The replication of positive-strand RNA viruses relies on virally encoded RNA-dependent RNA polymerases (RdRPs) that are capable of rapid and processive synthesis of the 7–14 kilobase viral genomes. To examine this in further detail and to validate the polymerase–RNA interactions seen in the initial poliovirus EC structures, we here present nine new coxsackievirus, rhinovirus, and poliovirus elongation complex structures at resolutions ranging from 2.1 to 2.9 Å. All the complexes feature an upstream RNA duplex that is pinched between the pinky finger and thumb domains such that the RNA exit channel is opened by ≈4 Å as compared to the polymerase alone structures. All of the complexes show the open conformation for the active site wherein the β-strands of motifs A and C are not hydrogen bonded together to fully form the RMM-fold that is commonly utilized by polymerase active sites.

Using this r2 RNA, we were able to obtain crystals of the CV polymerase EC under two conditions but in the same crystal form, resulting in a 2.4 Å resolution structure (CV_r2) and a 2.2 Å resolution structure (CV_r2_Mg) that clearly showed a Mg2+ ion pre-bound to the coxsackievirus polymerase EC in the absence of an added NTP. In the CV_r2_Mg structure we observe clear density for a six-fold coordinated magnesium ion bound to the polymerase at a site about 5 Å away from the active site itself. This is at a site that is commonly occupied by divalent metals in a number of other structures of the polymerase alone, and in several of the EC structures presented here the site is occupied by what is either a magnesium ion or a water molecule. In the CV_r2_Mg structure we see clear density for a bound magnesium ion that is coordinated by Asp330 in motif C and five water molecules in a six-fold coordination geometry, with Asp233 from motif A being involved in the network. This magnesium ion likely represents the polymerase bound Metal A ion that is moved into the active site to facilitate catalysis in conjunction with the Metal B magnesium that is brought in with the NTP, and it is bound in site where metals have been observed in several other viral polymerase structures even in the absence of RNA and NTPs.

>[4x]GEIEFIESSKDAGFPVINTPSKTKLEPSVFHQVFEGNKEPAVLRSGDPRLKANFEEAIFSKYIGNVNTHVDEYMLEAVDHYAGQLATLDISTEPMKLEDAVYGTEGLEALDLTTSAGYPYVALGIKKRDILSKKTKDLTKLKECMDKYGLNLPMVTYVKDELRSIEKVAKGKSRLIEASSLNDSVAMRQTFGNLYKTFHLNPGVVTGSAVGCDPDLFWSKIPVMLDGHLIAFDYSGYDASLSPVWFACLKMILEKLGYTHKETNYIDYLCNSHHLYRDKHYFVRGGMPSGCSGTSIFNSMINNIIIRTLMLKVYKGIDLDQFRMIAYGDDVIASYPWPIDASLLAEAGKGYGLIMTPADKGECFNEVTWTNVTFLKRYFRADEQYPFLVHPVMPMKDIHESIRWTKDPKNTQDHVRSLCLLAWHNGEHEYEEFIRKIRSVPVGRCLTLPAFSTLRRKWLDSFGSSSHHHHHH>MLGLKTSIIGRRVIYFQEITSTNEFAKTSYLEEGTVIVADKQTMGHGRLNRKWESPEGGLWLSIVLSPKVPQKDLPKIVFLGAVGVVETLKEFSIDGRIKWPNDVLVNYKGIAGVLVEGKGDKIVLGIGLNVNNKVPNGATS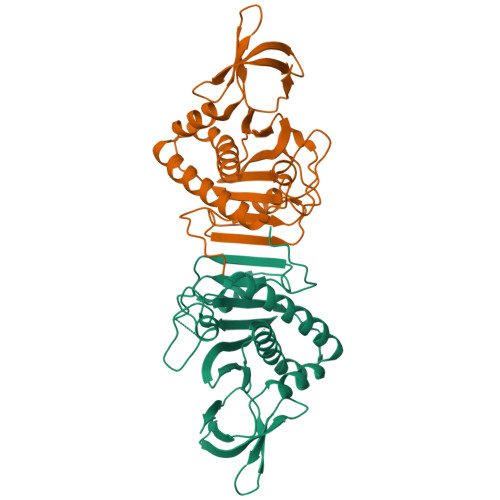MKLELGSEVPLLSVFRSLITNLDRLYLNFLKNPMDILNLVRDNMILGVRVKILGDGSFEGIAEDIDDFGRLIIRLDSGEVKKVIYGDVSLRFL[2x]> MKEYRSPELKEYGRV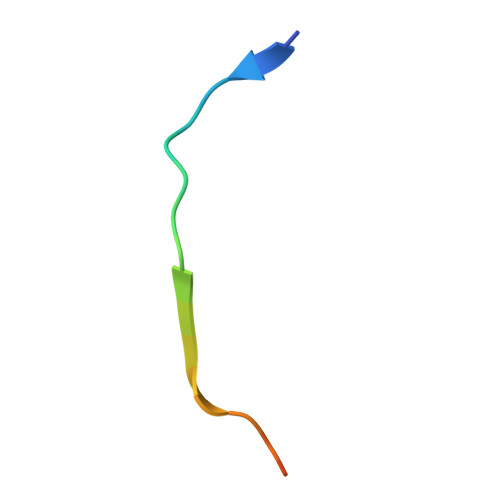EDRTAG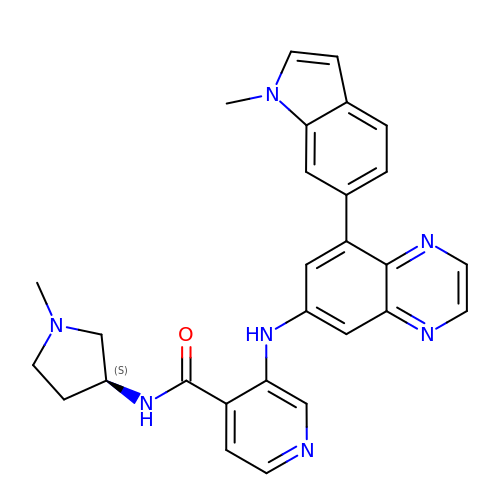3-[[8-(1-methylindol-6-yl)quinoxalin-6-yl]amino]-~{N}-[(3~{S})-1-methylpyrrolidin-3-yl]pyridine-4-carboxamide | C28 H27 N7 O | JQYNBBAXGSXALE-FQEVSTJZSA-N>MTMDEQQSQAVAPVYVGGFLARYDQSPDEAELLLPRD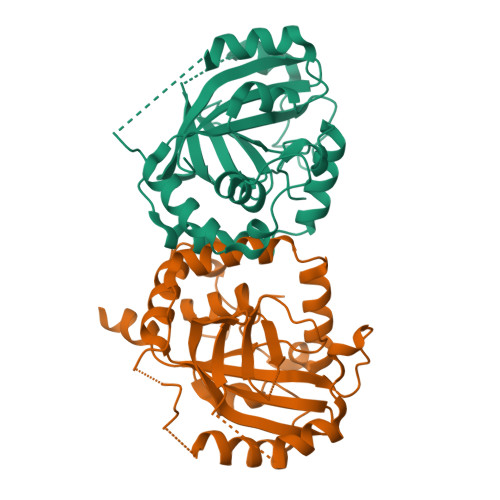VVEHWLHAQGQGQPSLSVALPLNINHDDTAVVGHVAAMQSVRDGLFCLGCVTSPRFLEIVRRASEKSELVSRGPVSPLQPDKVVEFLSGSYAGLSLSSRRCDDVEQATSLSGSETTPFKQVALCSVGRRRGTLAVYGRDPEWVTQRFPDLTAADRDGLRAQWQRCGSTAVDASGDPFRSDSYGLLGNSVDALYIRERLPKLRYDKQLVGVTERESYVKA[2x]> CGETCTLGTCY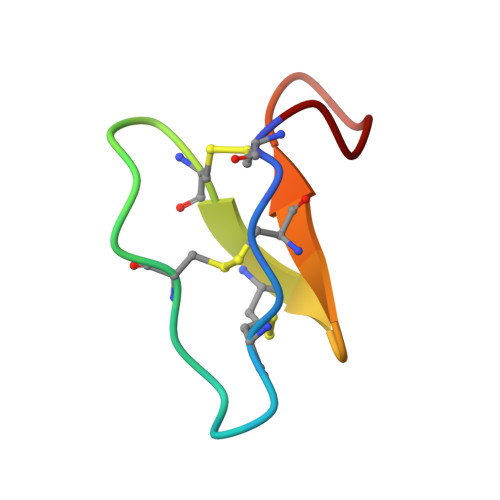TAGCSCSWPVCTRNGVPI> TRDQNGTWEMESNENFEG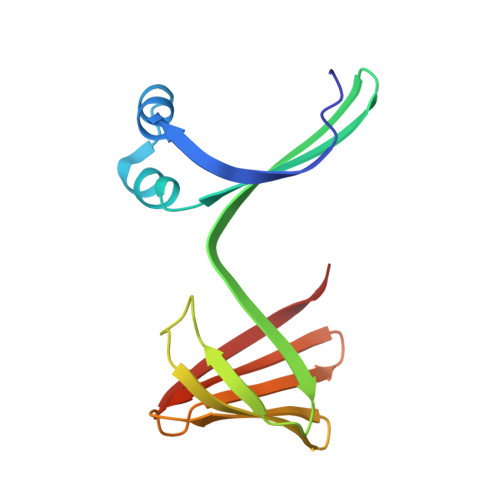YMKALDIDFATRKIAVRLTQTDVIDQDGDNFKTKTTSTFRNYDVDFTVGVEFDEYTKSLDNRHVKALVTWEGDVLVCVQKGEKENRGWKKWIEGDKLYLELTCGDQVCRQVFKKK>MGANASALEKEIGPEQFPVNEHYFGLVNFGNTCYCNSVLQALYFCRPFREKVLAYKS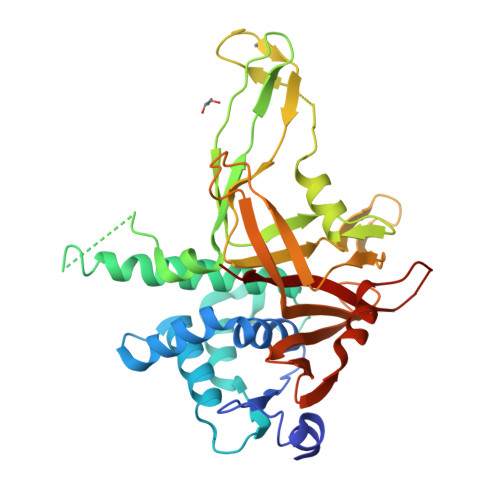QPRKKESLLTCLADLFHSIATQKKKVGVIPPKKFITRLRKENELFDNYMQQDAHEFLNYLLNTIADILQEERKQEKQNGRLPNGNIDNENNNSTPDPTWVHEIFQGTLTNETRCLTCETISSKDEDFLDLSVDVEQNTSITHCLRGFSNTETLCSEYKYYCEECRSKQEAHKRMKVKKLPMILALHLKRFKYMDQLHRYTKLSYRVVFPLELRLFNTSGDATNPDRMYDLVAVVVHCGSGPNRGHYIAIVKSHDFWLLFDDDIVEKIDAQAIEEFYGLTSDISKNSESGYILFYQSRD[2x]> KKRYDREFLL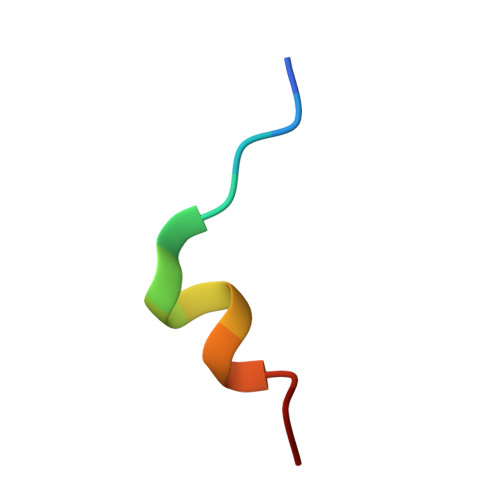GFQF>[4x]MGSDKIHHHHHHMKVVPAQRCVYSFSANMAPVEEVYPGEQVVFETLDALGGSYDKIDFSKVNPATGPVFVNGVKPGDTLKVRIKRIELPRRGMIVTGKGFGVLGDEVEGFHTKELEIEKWAVLFDGVRIPIHPMVGVIGVAPQEGEYPTG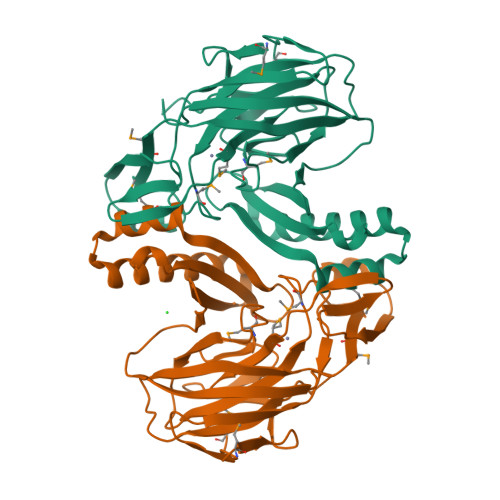TAHRHGGNMDTKEITENVTVHLPVFQEGALLALGDVHATMGDGEVCVSACEVPAKVVVEIDVSKEEIKWPVVETNDAYYIIVSLPDIEEALKEVTRETVWFIQRRKTIPFTDAYMLASLSVDVGISQLVNPAKTAKARIPKYIFTGV> MAMQAAKRANIRLPPEVNRILYIRNLPYKITAEEMYDIFGKYGPIRQIRVGNTPETRGTAYVVYEDIFDAKNACDHLSGFNVCNRYLVVLYYNANRAFQKMDTKKKEEQLKLLKEKYGINTDP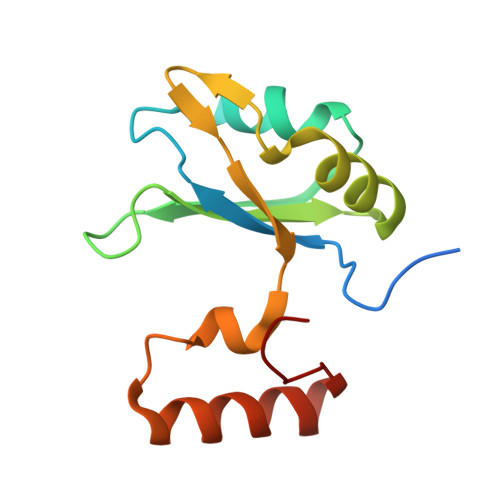PK> NLYQFKNMIQCTVPSRSWADFADYGCYCGKGGSGTPVDDLDRCCQTHDNCYNEAENISGCRPYFKTYSYECTQ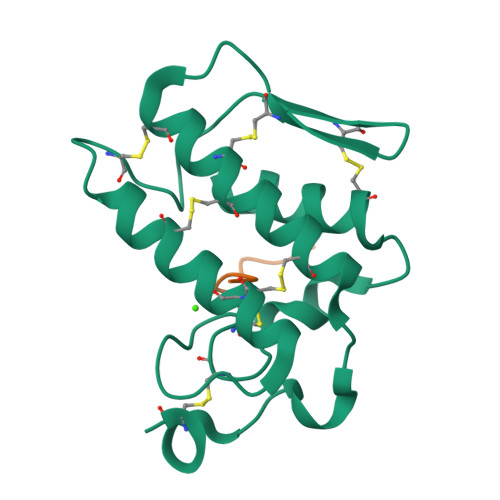GTLTCKGDNNACAASVCDCDRLAAICFAGAPYNDANYNIDLKARCN;> DAEFRHDS>MSLTETQSLELAKELISRPSVTPDDRDCQKLMAERLHKIGFAAEEMHFGNTKNIWLRRGTKAPVVCFAGHTDVVPTGPVEKWDSPPFEPAERDGRLYGRGAADMKTSIACFVTACERFVAKHPNHQGSIALLITSDEEGDALDGTTKVVDVLKARDELIDYCIVGEPTAVDKLGDMIKNGRRGSLSGNLTVKGKQGHIAYPHLAINPVHTFAPALLELTQEVWDEGNEYFPPTSFQISNINGGTGATNVIPGELNVKFNFRFSTESTEAGLKQRVHAILDKHGVQYDLQWSCSGQPFLTQAGKLTDVARAAI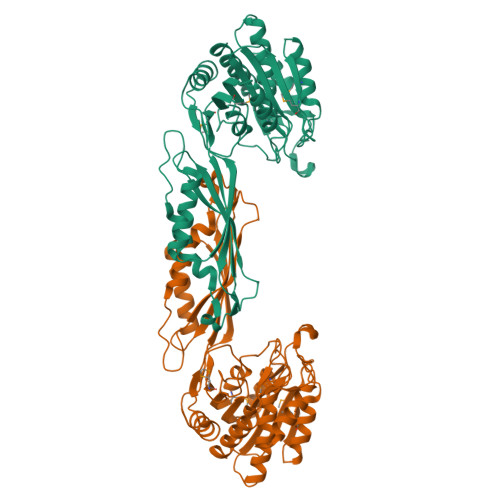AETCGIEAELSTTGGTSDGRFIKAMAQELIELGPSNATIHQINENVRLNDIPKLSAVYEGILVRLLAGNAVEGGSHHHHHH[2x]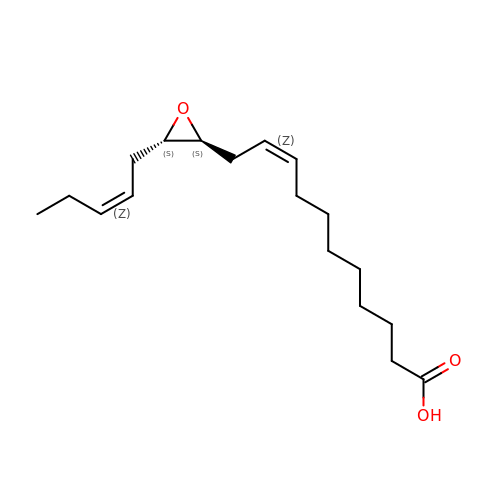(9Z)-11-{(2S,3S)-3-[(2Z)-pent-2-en-1-yl]oxiran-2-yl}undec-9-enoic acid | C18 H30 O3 | BKKGUKSHPCTUGE-WXDGQRKDSA-N>[2x]PGHMKTVLMVAEKPSLAQSIAKILSRGSLSSHKGLNGACSVHEYTGTFAGQPVRFKMTSVCGHVMTLDFLGKYNKWDKVDPAELFSQAPTEKKEANPKLNMVKFLQVEGRGCDYIVLWLDCDKEGENICFEVLDAVLPVMNKAHGGEKTVFRARFSSITDTDICNAMACLGEPDHNEALSVDARQELDLRIGCAFTRFQTKYFQGKYGDLDSSLISFGPCQTPTLG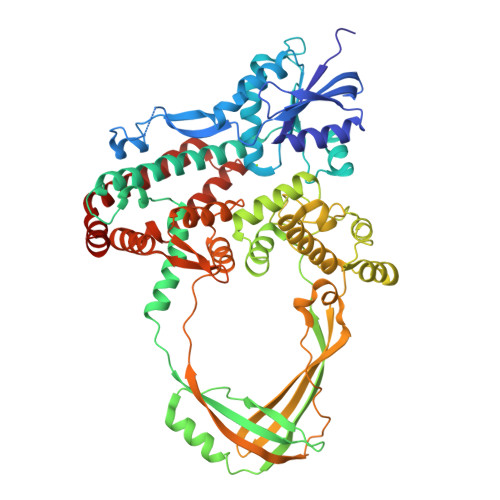FCVERHDKIQSFKPETYWVLQAKVNTDKDRSLLLDWDRVRVFDREIAQMFLNMTKLEKEAQVEATSRKEKAKQRPLALNTVEMLRVASSSLGMGPQHAMQTAERLYTQGYISYPRTETTHYPENFDLKGSLRQQANHPYWADTVKRLLAEGINRPRKGHDAGDHPPITPMKSATEAELGGDAWRLYEYITRHFIATVSHDCKYLQSTISFRIGPELFTCSGKTVLSPGFTEVMPWQSVPLEESLPTCQRGDAFPVGEVKMLEKQTNPPDYLTEAELITLMEKHGIGTDASIPVHINNICQRNYVTVESGRRLKPTNLGIVLVHGYYKIDAELVLPTIRSAVEKQLNLIAQGKADYRQVLGHTLDVFKRKFHYFVDSIAGMDELMEVSFS> PNFSGNWKIIRSENFEELLKVLGVNVMLRKIWVAAASKPAVEIKQEGDTF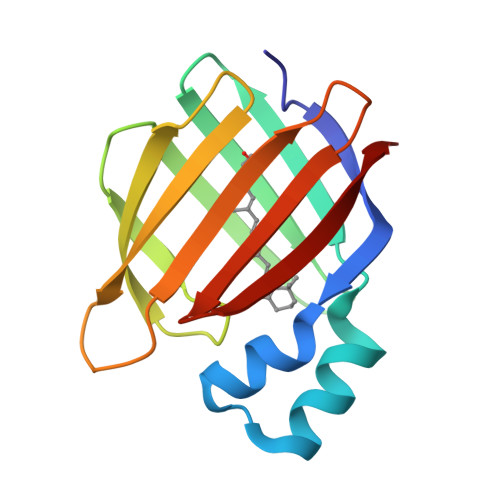YIKVSTTVWTTEINFKVGEEFEEQTVDGRPCKSLVKWESENKMVCEQKLLKGEGPKTSWTKELTNDGELILTMTADDVVCTQVFVRE> GPVEESVERAMVRVADTVSSKPTNSESIPALTAAETGHTSQVVPSDTMQTRHVKNYHSRSESSIENFLCRSACVYYATYNNNSEKGYAEWVINTRQVAQLLRRKLEFTYLRFDLELTFVITSAQEPSTATSVDAPVQTQQIMYVPPGGPVPTKVTDYAWQTSTNPSVFWTEGNAPPRMSIPFISIGNAYSCFYDGWTQ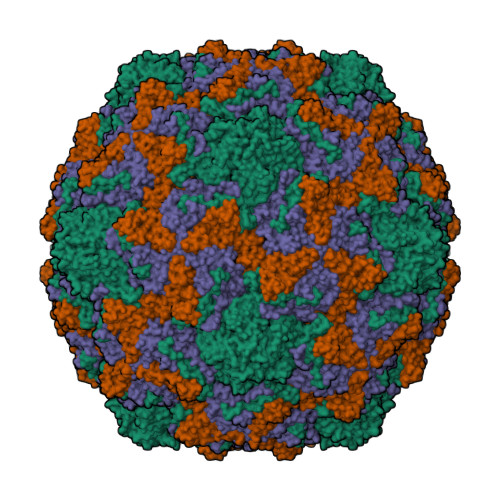FSRNGVYGINTLNNMGTLYMRHVNEAGQGPIKSTVRIYFKPKHVKAWVPRPPRLCQYEKQKNVNFNPTGVTTTRSNITTT;> SPSAEECGYSDRVRSITLGNSTITTQECANVVVGYGVWPEYLKDNEATGEDQPTQPDVATCRFYTLESVQWMKNSAGWWWKLPDALSQMGLFGQNMQYHYLGRTGYTIHVQCNASKFHQGCLLVVCVPEAEMGCSNLNNTPKFAELSGGDNARMFTDTEVGTSNDKKVQTAVWNAGMGVGVGNLTIFPHQWINLRTNNSATIVMPYINSVPMDNMYRHNNLTLMIIPFVPLNYSEGSSPYVPITVTIAPMCAEYNGLRLASSQ;> GLPVMTTPGSTQFLTSDDFQSPSAMPQFDVTPEMQIPGRVNNLMEIAEVDSVVPVNNTDNNVNGLKAYQIPVQSNSDNRRQVFGFPLQPGANNVLNRTLLGEILNYYTHWSGSIKLTFMFCGSAMATGKFLLAYSPPGAGVPKNRRDAMLGTHVIWDVGLQSSCVLCVPWISQTHYRYVVEDEYTAAGYVTCWYQTNIIVPADVQSTCDILCFVSACNDFSVRMLKDTPFIRQDNFYQ;> GAQVSTQKTGAHETGLNASGNSIIHYTNINYYKDAASNSANRQDFTQDPGKFTEPVKDIMIKSMPALN>[3x]KEVKIGMAIDDLRLERWQKDRDIFVKKAESLGAKVFVQSANGNEETQMSQIENMINRGVDVLVIIPYNGQVLSNVVKEAKQEGIKVLAYDRMINDADIDFYISFDNEKVGELQAKALVDIVPQGNYFLMGGSPVDNNAKLFRAGQMKVLKPYVDS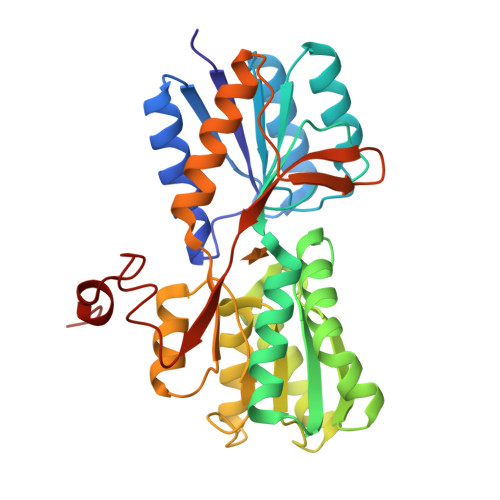GKIKVVGDQWVDGWLPENALKIMENALTANNNKIDAVVASNDATAGGAIQALSAQGLSGKVAISGQDADLAGIKRIAAGTQTMTVYKPITLLANTAAEIAVELGNGQEPKADTTLNNGLKDVPSRLLTPIDVNKNNIKDTVIKDGFHKESELHHHHHH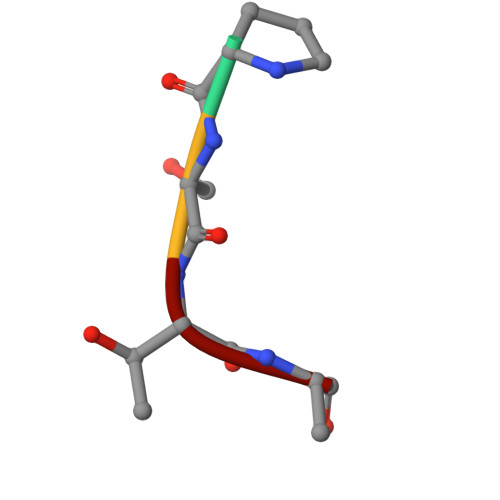> PSTA[(3R,5R,6S)-1-[(2S)-1-tert-butoxy-1-oxobutan-2-yl]-5-(3-chlorophenyl)-6-(4-chlorophenyl)-2-oxopiperidin-3-yl]acetic acid | C27 H31 Cl2 N O5 | 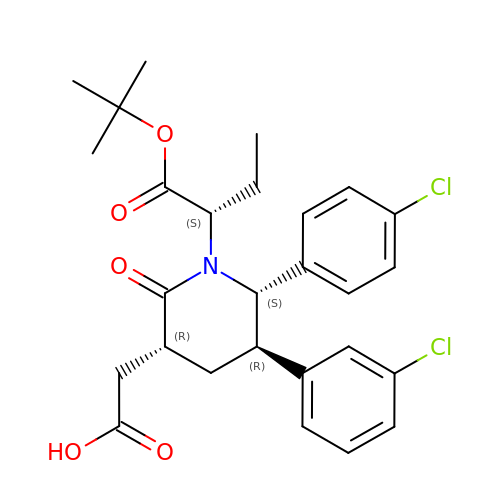ZEMLYWMOSZRCQL-UWSZBUKDSA-N> MSENTVMPIVRVAVLAAGDDGGRLTEMALPSELPLREILPAVQRIVQPARENDGAADPAAAPNPVRLSLAPIGGAPFSLDATLDTVGVVDGDLLALQAVPSGPPAPRIVEDIADAAVIFSEARRRQWGPTHIARGAALALIGLILVGTGLSVAHRVITGDLLGQFIVSGIALATVIAALAVRNRSAVLATSLAVTALVPVAAAFALGVPGDFGAPNVLLAAAGVAAWSLISMAGSPDDRGIAVFTATAVTGVGVLLVAGAASLWVISSDVIGCALVLLGLIVTVQAAQLSAMWARFPLPVIPAPGDPTPAARPLSVLADLPRRVRVSQAHQTGVIAAGVLLGVAGSVALVSSANASPWAWYIVVAA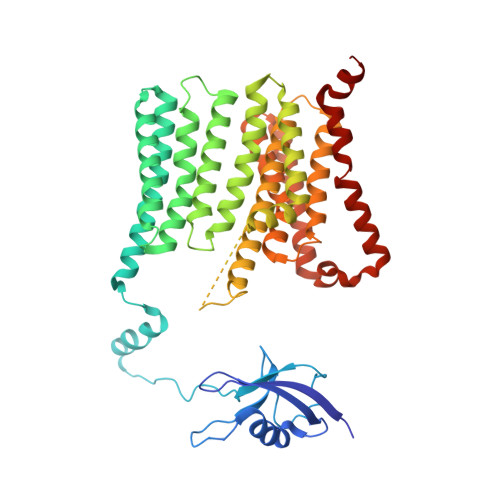AAGAALRARVWDSAACKAWLLGHSYLLAVALLVAFVIGDRYQAALWALAALAVLVLVWIVAALNPKIASPDTYSLPMRRMVGFLATGLDASLIPVMALLVGLFSLVLDR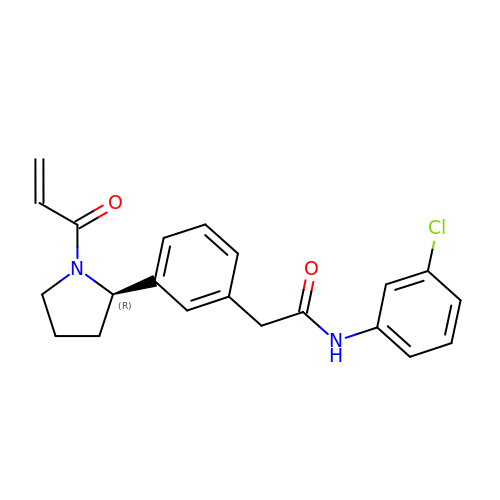2-{3-[(2R)-1-acryloylpyrrolidin-2-yl]phenyl}-N-(3-chlorophenyl)acetamide | C21 H21 Cl N2 O2 | HVSHMSOMUBRQOZ-LJQANCHMSA-N>GSTGSMFKLLLIFADPAEAARTLSLFPFSLNKENFYTYHTENVLLDVMVLKTWGYRGVVQALSPPPSGYDLWINAGFAGAANPNIPLLKTYTITSVKELTPTTSVEEELEVTPIPRLPLAQLTSVRSPYRDGFHEHLQLVDMEGFFIAKQASLVACPCSMIKVSSDYTT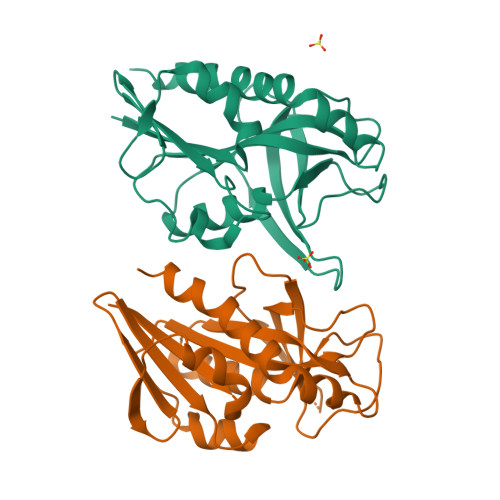REGQDFLKNNKVKLSQKLAEAIFPIYSSFIDV[2x]Parkin is an RBR-type ubiquitin ligase which is characterized by RING1, inBetweenRING (IBR) and RING2 domains. Parkin has an N-terminal ubiquitin-like domain (Ubl) that shares 65% sequence similarity with ubiquitin, and a zinc-chelating RING0 domain immediately N-terminal to the RBR domains (Hristova et al, 2009). The RING1 domain recruits E2 enzymes, which carry charged ubiquitin and pass it to a catalytic cysteine in the parkin RING2 domain (Wenzel et al, 2011). Wild-type parkin exists in an autoinhibited state (Chaugule et al, 2011); subsequently, autoinhibition has been demonstrated to be common to RBR ligases (Smit et al, 2012; Stieglitz et al, 2012; Duda et al, 2013).

In particular, one construct (UblR0RBR) that included the Ubl (residues 1–83) linked to RING0RBR (residues 144–465) showed autoinhibition similar to the wild-type protein, enhanced ubiquitination with phosphoubiquitin and the ability to ubiquitinate a potential mitochondrial substrate protein, Miro1 (Kazlauskaite et al, 2014a) (Fig1B). The crystal structure of UblR0RBR parkin was solved and refined to 1.8 Å, and comprises two molecules in the asymmetric unit. The structure has five domains: Ubl (1–76), RING0 (144–216), RING1 (228–327), IBR (328–377) and RING2 (415–465), and a repressor element (REP) (Fig1C). The largest interface in the structure is that formed between the Ubl domain and the rest of parkin, burying ∼2,150 Å2 accessible surface area (Fig2A). The primary contact is between the Ubl (β3, β5) and RING1 (helix H1) domains (Fig2A; Fig EV1). The core interface is stabilized by hydrophobic interactions mediated by I44 and V70 of the Ubl domain and L266, V269 and T270 of RING1 (Fig2A). This interaction is supported by several key salt bridges and hydrogen bonds including R42 (Ubl) with D262 at the N-terminus of helix H1 (RING1) and R6 and H68 (Ubl) with N273 and D274 at the C-terminus of helix H1. In UblR0RBR, the RING0/RING1 interface buries 730 Å2 and involves Y147, Y149, K151, Q155, V157, W183 and L187 of the RING0 domain interacting with H227, I229, A230, P247, E300, H302, R305, I306 and E309 of the RING1 domain (Figs3B and EV1). A salt bridge formed by R234 and E404 pinning the domains together is absent in the R0RBR structure, but present when the Ubl domain is attached. In the Ubl-bound structure, the side chains of H302 and E300 (and H227) are facing into the interface, while in the R0RBR structures, these residues are flipped out ∼180° away from the interface (Fig3C).

>[2x]MIVFVRFNSSHGFPVEVDSDTSIFQLKEVVAKRQGVPADQLRVIFAGKELRNDWTVQNCDLDQQSIVHIVQRPWRKGQEMNATNSFYVYCKGPCQRVQPGKLRVQCSTCRQATLTLTQGPSCWDDVLIPNRMSGECQSPHCPGTSAEFFFKCGAHPTSDKETSVALHLIATNSRNITCITCTDVRSPVLVFQCNSRHVICLDCFHLYCVTRLNDRQFVHDPQLGYSLPCVAGCPNSLIKELHHFRILGEEQYNRYQQYGAEECVLQMGGVLCPRPGCGAGLLPEPDQRKVTCEGGNGLGCGFAFCRECKEAYHEGECSAVFEASGTTTQAYRVDERAAEQARWEAASKETIKKTTKPCPRCHVPVEKNGGCMHMKCPQPQCRLEWCWNCGCEWNRVCMGDHWFDV> MAHHHHHHGMTRTRSGSLAAGGLNWASLPLKLFAGGNAKFWHPAD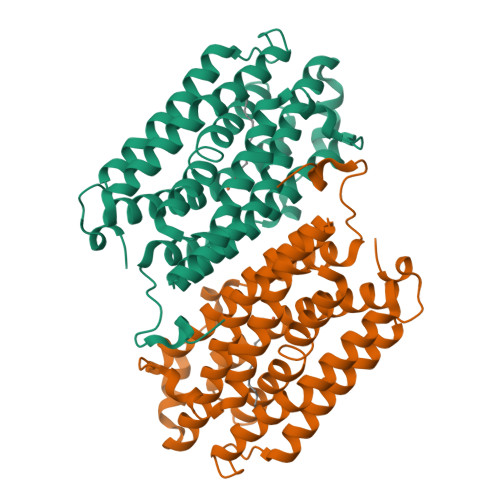IDFTRDRADWEKLSDDERDYATRLCTQFIAGEEAVTEDIQPFMSAMRAEGRLADEMYLTQFAFEEAKHTQVFRMWLDAVGISEDLHRYLDDLPAYRQIFYAELPECLNALSADPSPAAQVRASVTYNHIVEGMLALTGYYAWHKICVERAILPGMQELVRRIGDDERRHMAWGTFTCRRHVAADDANWTVFETRMNELIPLALRLIEEGFALYGDQPPFDLSKDDFLQYSTDKGMRRFGTISNARGRPVAEIDVDYSPAQLEDTFADEDRRTLAAASA> MLEQPYLDLAKKVLDEGHFKPDRTHTGTYSIFGHQMRFDLSKGFPLLTTKKVPFGLIKSQLLWFLHGDTNIRFLLQHRNHIWDEWAFEKWVKSDEYHGPDMTDFGHRSQKAPEFAAVYHEEMAKFDDRVLHDDAFAAKYGDLGLVYGSQWRAWHTSKGDTIDQLGDVIE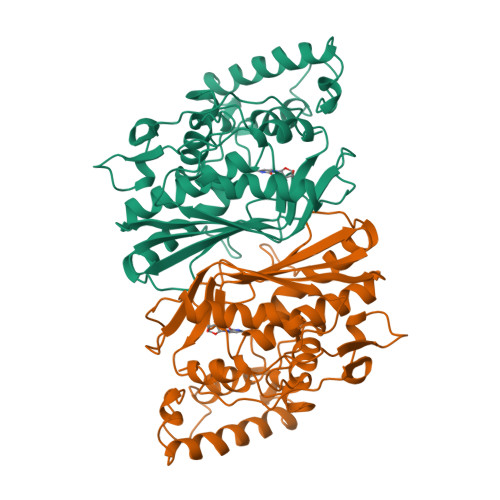QIKTHPYSRRLIVSAWNPEDVPTMALPPCHTLYQFYVNDGKLSLQLYQRSADIFLGVPFNIASYALLTHLVAHECGLEVGEFIHTFGDAHLYVNHLDQIKEQLSRTPRPAPTLQLNPDKHDIFDFDMKDIKLLNYDPYPAIKAPVAV Clathrin-mediated endocytosis (CME) is a vital multistep process in all eukaryotes in which plasma membrane cargo proteins are first concentrated into a patch by clathrin adaptors, which are themselves clustered by interaction with a polymeric clathrin scaffold. The most abundant clathrin adaptor is the 300-kDa heterotetrameric adaptor protein 2 (AP2) complex, consisting of α, β2, μ2, and σ2 subunits. AP2 plays a central role in CME through binding plasma membrane phosphatidylinositol 4,5-bisphosphate [PtdIns(4,5)P2], the two most common cargo motifs (YxxΦ and [ED]xxxL[LI]), clathrin, and other regulatory/accessory proteins [reviewed in (1)]. Here, we used cryo–electron microscopy, tomography, and subtomogram averaging to determine structures, interactions, and arrangements of clathrin and AP2 at the key steps of coat assembly, from AP2 in solution to membrane-assembled clathrin-coated vesicles (CCVs).

We determined the structure of clathrin above AP2 in both the YxxΦ and YxxΦ/[ED]xxxL[LI] cargo–containing liposomes by subtomogram averaging: The structures were the same and thus were combined for further analysis. The CLC region that contacts CHC is well resolved, as are most of the leg and the helical hub of CHC. The resolution is lower toward the NTDs of CHC that extend downward toward the membrane, reflecting mobility of these domains, but is sufficient to position the full NTD. Our structures are generally consistent with those previously described from purified clathrin in solution in the absence of membranes, but by now resolving the NTDs, we were able to derive the positions of peptide-binding sites within the clathrin cage. Between the clathrin NTDs and the undersides of the triskelia, we observed a “bean-shaped” density that is not part of clathrin. β2 appendages link CHC repeat 1 in one clathrin molecule, CHC repeat 2 in a second clathrin molecule (both in the ankle region), and the NTD of a third clathrin molecule. This positions the β2 appendage such that its C-terminal platform subdomain is freely accessible to the Fxx[FL]xxxR helical motifs on the unstructured portions of secondary adaptors such as autosomal recessive hypercholesterolemia (ARH) protein, arrestins, and epsins rather than being blocked as speculated. Another motif-binding site, recognized by regulatory/accessory proteins including Eps15, is located on the β2 appendage sandwich domain close to the point of interaction with CHC repeat 2. We now see that auxilin would occupy a cavity bounded by the β2 appendage, an NTD, and clathrin ankles.

>[8x]MAQILPIRFQEHLQLQNLGINPANIGFSTLTMESDKFICIREKVGEQAQVVIIDMNDPSNPIRRPISADSAIMNPASKVIALKAGKTLQIFNIEMKSKMKAHTMTDDVTFWKWISLNTVALVTDNAVYHWSMEGESQPVKMFDRHSSLAGCQIINYRTDAKQKWLLLTGISAQQNRVVGAMQLYSVDRKVSQPIEGHAASFAQFKMEGNAEESTLFCFAVRGQAGGKLHIIEVGTPPTGNQPFPKKAVDVFFPPEAQNDFPVAMQISEKHDVVFLITKYGYIHLYDLETGTCIYMNRISGETIFVTAPHEATAGIIGVNRKGQVLSVCVEEENIIPYITNVLQNPDLALRMAVRNNLAGAEELFARKFNALFAQGNYSEAAKVAANAPKGILRTPDTIRRFQSVPAQPGQTSPLLQYFGILLDQGQLNKYESLELCRPVLQQGRKQLLEKWLKEDKLECSEELGDLVKSVDPTLALSVYLRANVPNKVIQCFAETGQVQKIVLYAKKVGYTPDWIFLLRNVMRISPDQGQQFAQMLVQDEEPLADITQIVDVFMEYNLIQQCTAFLLDALKNNRPSEGPLQTRLLEMNLMHAPQVADAILGNQMFTHYDRAHIAQLCEKAGLLQRALEHFTDLYDIKRAVVHTHLLNPEWLVNYFGSLSVEDSLECLRAMLSANIRQNLQICVQVASKYHEQLSTQSLIELFESFKSFEGLFYFLGSIVNFSQDPDVHFKYIQAACKTGQIKEVERICRESNCYDPERVKNFLKEAKLTDQLPLIIVCDRFDFVHDLVLYLYRNNLQKYIEIYVQKVNPSRLPVVIGGLLDVDCSEDVIKNLILVVRGQFSTDELVAEVEKRNRLKLLLPWLEARIHEGCEEPATHNALAKIYIDSNNNPERFLRENPYYDSRVVGKYCEKRDPHLACVAYERGQCDLELINVCNENSLFKSLSRYLVRRKDPELWGSVLLESNPYRRPLIDQVVQTALSETQDPEEVSVTVKAFMTADLPNELIELLEKIVLDNSVFSEHRNLQNLLILTAIKADRTRVMEYINRLDNYDAPDIANIAISNELFEEAFAIFRKFDVNTSAVQVLIEHIGNLDRAYEFAERCNEPAVWSQLAKAQLQKGMVKEAIDSYIKADDPSSYMEVVQAANTSGNWEELVKYLQMARKKARESYVETELIFALAKTNRLAELEEFINGPNNAHIQQVGDRCYDEKMYDAAKLLYNNVSNFGRLASTLVHLGEYQAAVDGARKANSTRTWKEVCFACVDGKEFRLAQMCGLHIVVHADELEELINYYQDRGYFEELITMLEAALGLERAHMGMFTELAILYSKFKPQKMREHLELFWSRVNIPKVLRAAEQAHLWAELVFLYDKYEEYDNAIITMMNHPTDAWKEGQFKDIITKVANVELYYRAIQFYLEFKPLLLNDLLMVLSPRLDHTRAVNYFSKVKQLPLVKPYLRSVQNHNNKSVNESLNNLFITEEDYQALRTSIDAYDNFDNISLAQRLEKHELIEFRRIAAYLFKGNNRWKQSVELCKKDSLYKDAMQYASESKDTELAEELLQWFLQEEKRECFGACLFTCYDLLRPDVVLETAWRHNIMDFAMPYFIQVMKEYLTKVDKLDASESLRKEEEQATETQ;> MAQILPIRFQEHLQLQNLGINPANIGFSTLTMESDKFICIREKVGEQAQVVIIDMNDPSNPIRRPISADSAIMNPASKVIALKAGKTLQIFNIEMKSKMKAHTMTDDVTFWKWISLNTVALVTDNAVYHWSMEGESQPVKMFDRHSSLAGCQIINYRTDAKQKWLLLTGISAQQNRVVGAMQLYSVDRKVSQPIEGHAASFAQFKMEGNAEESTLFCFAVRGQAGGKLHIIEVGTPPTGNQPFPKKAVDVFFPPEAQNDFPVAMQISEKHDVVFLITKYGYIHLYDLETGTCIYMNRISGETIFVTAPHEATAGIIGVNRKGQVLSVCVEEENIIPYITNVLQNPDLALRMAVRNNLAGAEELFARKFNALFAQGNYSEAAKVAANAPKGILRTPDTIRRFQSVPAQPGQTSPLLQYFGILLDQGQLNKYESLELCRPVLQQGRKQLLEKWLKEDKLECSEELGDLVKSVDPTLALSVYLRANVPNKVIQCFAETGQVQKIVLYAKKVGYTPDWIFLLRNVMRISPDQGQQFAQMLVQDEEPLADITQIVDVFMEYNLIQQCTAFLLDALKNNRPSEGPLQTRLLEMNLMHAPQVADAILGNQMFTHYDRAHIAQLCEKAGLLQRALEHFTDLYDIKRAVVHTHLLNPEWLVNYFGSLSVEDSLECLRAMLSANIRQNLQICVQVASKYHEQLSTQSLIELFESFKSFEGLFYFLGSIVNFSQDPDVHFKYIQAACKTGQIKEVERICRESNCYDPERVKNFLKEAKLTDQLPLIIVCDRFDFVHDLVLYLYRNNLQKYIEIYVQKVNPSRLPVVIGGLLDVDCSEDVIKNLILVVRGQFSTDELVAEVEKRNRLKLLLPWLEARIHEGCTEPATHNALAKIYIDSNNNPERFLRENPYYDSRVVGKYCEKRDPHLACVAYERGQCDLELINVCNENSLFKSLSRYLVRRKDPELWGSVLLESNPYRRPLIDQVVQTALSETQDPEEVSVTVKAFMTADLPNELIELLEKIVLDNSVFSEHRNLQNLLILTAIKADRTRVMEYINRLDNYDAPDIANIAISNELFEEAFAIFRKFDVNTSAVQVLIEHIGNLDRAYEFAERCNEPAVWSQLAKAQLQKGMVKEAIDSYIKADDPSSYMEVVQAANTSGNWEELVKYLQMARKKARESYVETELIFALAKTNRLAELEEFINGPNNAHIQQVGDRCYDEKMYDAAKLLYNNVSNFGRLASTLVHLGEYQAAVDGARKANSTRTWKEVCFACVDGKEFRLAQMCGLHIVVHADELEELINYYQDRGYFEELITMLEAALGLERAHMGMFTELAILYSKFKPQKMREHLELFWSRVNIPKVLRAAEQAHLWAELVFLYDKYEEYDNAIITMMNHPTDAWKEGQFKDIITKVANVELYYRAIQFYLEFKPLLLNDLLMVLSPRLDHTRAVNYFSKVKQLPLVKPYLRSVQNHNNKSVNESLNNLFITEEDYQALRTSIDAYDNFDNISLAQRLEKHELIEFRRIAAYLFKGNNRWKQSVELCKKDSLYKDAMQYASESKDTELAEELLQWFLQEEKRECFGACLFTCYDLLRPDVVLETAWRHNIMDFAMPYFIQVMKEYLTKVDKLDASESLRKEEEQATETQ;>[4x]MADDFGFFSSSESGAPEVAEEDPAAAFLAQQESEIAGIENDEGFGAPAGSQAALAQPGPASGAGPEDMGTTVNGDVFQDANGPADGYAAIAQADRLTQEPESIRKWREEQRKRLQELDAASKVTEQEWREKAKKDLEEWNQRQSEQVEKNKINNRIADKAFYQQPDADIIGYVASEEAFVKESKEETPGTEWEKVAQLCDFNPKSSKQCKDVSRLRSVLMSLKQTPLSR;> GGYVAPKAVWLPAVKAKGLEISGTFTHRQGHIYMEMNFTNKALQHMTDFAIQFNKNSFGVIPSTPLAIHTPLMPNQSIDVSLPLNTLGPVMKMEPLNNLQVAVKNNIDVFYFSCLIPLNVLFVEDGKMERQVFLATWKDIPNENELQFQIKECHLNADTVSSKLQNNNVYTIAKRNVEGQDMLYQSLKLTNGIWILAELRIQPGNPNYTLSLKCRAPEVSQYIYQVYDSILKN4-{(1E)-3-OXO-3-[(2-PHENYLETHYL)AMINO]PROP-1-EN-1-YL}-1,2-PHENYLENE DIACETATE 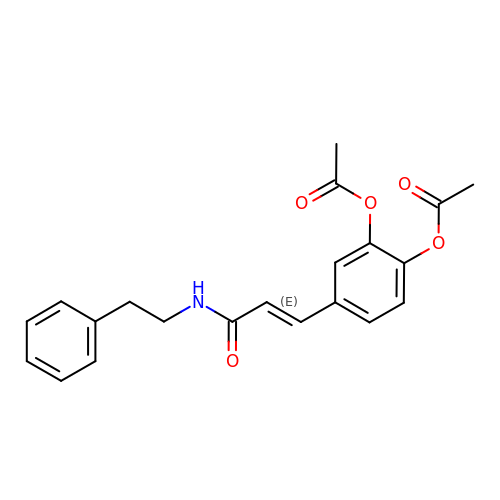| C21 H21 N O5 | GARHCDOTUULBOQ-PKNBQFBNSA-N>[2x]GEILKELPEGFDKETVRKQAMEDIEIAQSKDYESWKSRFTKDLQSSL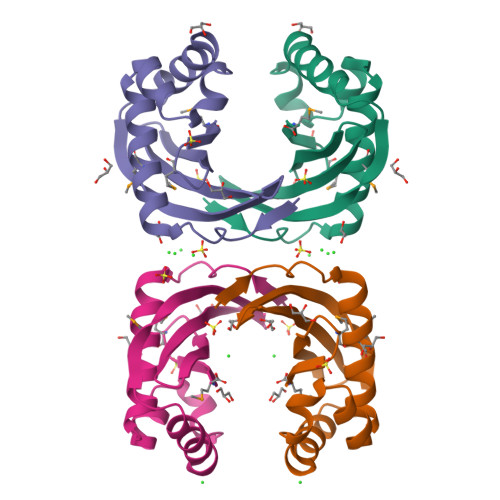TEESYDSYLKILEKQGEFKEFGKCTYLGQIKDNKKYGGVIIVVKYEEGNVNYSLAYDEDMNLVSFTM>MCTGLALETKDGLHLFGRNMDIEYSFNQSIIFIPRNFKCVNKSNKKELTTKYAVLGMGTIFDDYPTFADGMNEKGLGCAGLNFPVYVSYSKEDIEGKTNIPVYNFLLWVLANFSSVEEVKEALKNANIVDIPISENIPNTTLHWMISDITGKSIVVEQTKEKLNVFDNNIGVLTNSPTFDWHVANLNQYVGLRYNQVPEFKLGDQSLTALGQGTGLVGLPGDFTPASRFIRVAFLRDAMIKNDKDSIDLIEFFHILNNVAMVRGSTRTVEEKSDLTQYTSCMCLEKGIYYYNTYENNQINAIDMNKENLDGNEIKTYKYNKTLSINH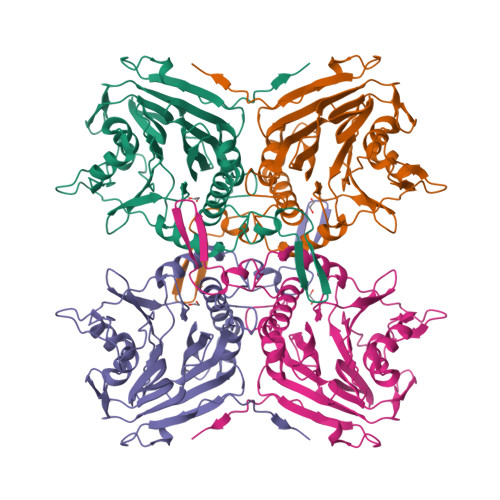VN[2x]(6-phenyl-1-benzofuran-3-yl)acetic acid 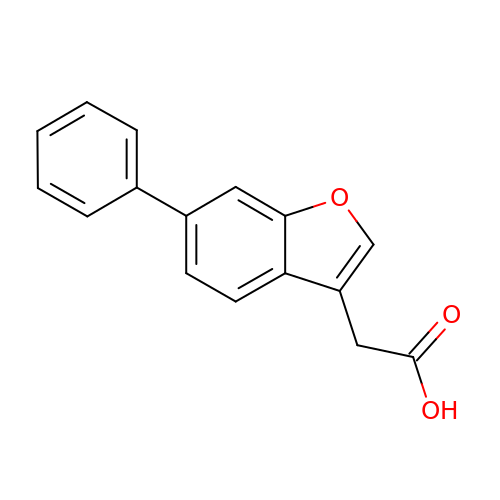| C16 H12 O3 | UIXZLSWUYGJHOL-UHFFFAOYSA-N>XSLSDKDKAAVRALWSKIGKSADAIGNDALSRMIVVYPQ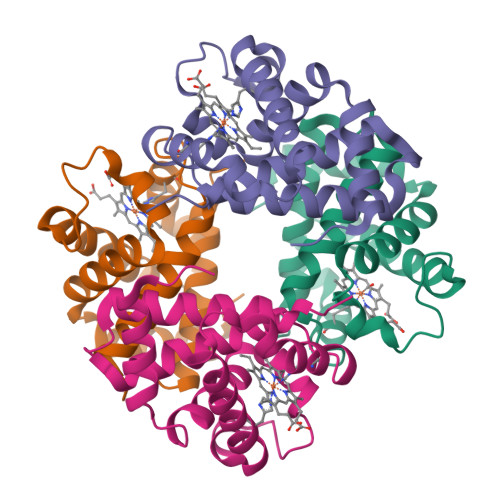TKTYFSHWPDVTPGSPHIKAHGKKVMGGIALAVSKIDDLKTGLMELSEQHAYKLRVDPANFKILNHCILVVISTMFPKEFTPEAHVSLDKFLSGVALALAERYR[2x];>[2x]VEWTDKERSIISDIFSHMDYDDIGPKALSRCLIVYPWTQRHFSGFGNLYNAEAIIGNANVAAHGIKVLHGLDRGVKNMDNIAATYADLSTLHSEKLHVDPDNFKLLSDCITIVLAAKMGHAFTAETQGAFQKFLAVVVSALGKQYH>[3x]MERLDIFGVPIDRVTMIQAVDIL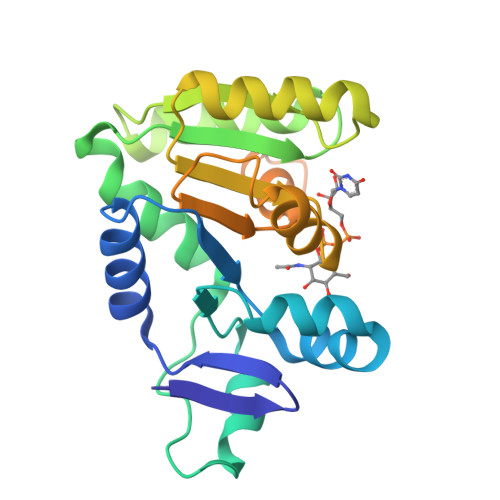NNFLQENRLHIVATPNAEIVMMAQKDKEYMEILNNTDLNVPDGSGIVFASKVFKKPLPERVAGFDLMLEFIKGISSKGVKIYLLGAAAQVAEQARANLEKLYPGVKIVGTHHGYFTEEEENKIIEEINNKGAEVLFVALGAPKQEKWIYKNKDKLKVKIAMGVGGSFDVIAGKVKRAPYEYRKLGQEWKYRLEKEPWRYKRMMALPKFAIKVLLHKREVVR>[2x]ATQGQVITCKAAVAYEPNKPLVIEDVQVAPPQAGEVRIKILYTALCHTDAYTWSGKDPEGLFPCILGHEAAGIVESVGEGVTEVQAGDHV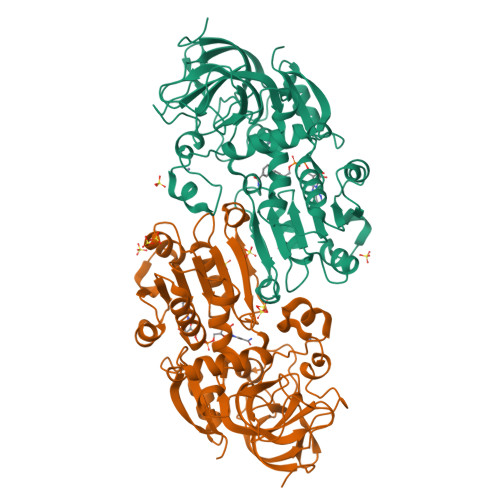IPCYQAECRECKFCKSGKTNLCGKVRSATGVGIMMNDRKSRFSVNGKPIYHFMGTSTFSQYTVVHDVSVAKIDPTAPLDKVCLLGCGVPTGLGAVWNTAKVEPGSNVAIFGLGTVGLAVAEGAKTAGASRIIGIDIDSKKYETAKKFGVNEFVNPKDHDKPIQEVIVDLTDGGVDYSFECIGNVSVMRAALECCHKGWGTSVIVGVAASGQEISTRPFQLVTGRVWKGTAFGGFKSRTQVPWLVEKYMNKEIKVDEYITHNLTLGEINKAFDLLHEGTCLRCVLDTSK> AKVEVGDEVGNFKFYPDSITVSAGEAVEFTLVGETGHNIVFDIPAGAPGTVASELKAASMDENDLLSEDEPS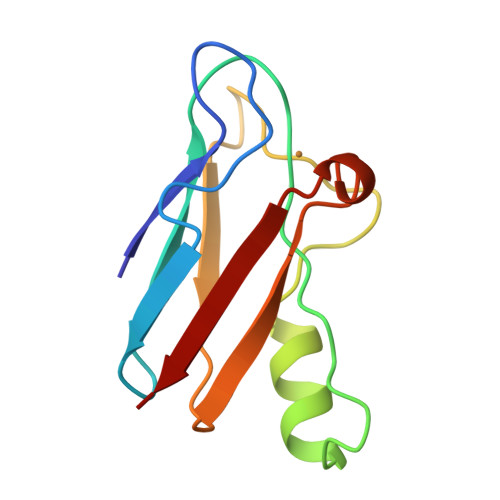FKAKVSTPGTYTFYCTPHKSANMKGTLTVK>[2x]MEICPAVKRDVDLFLTGTPDEYVEQVAQYKALPVVLE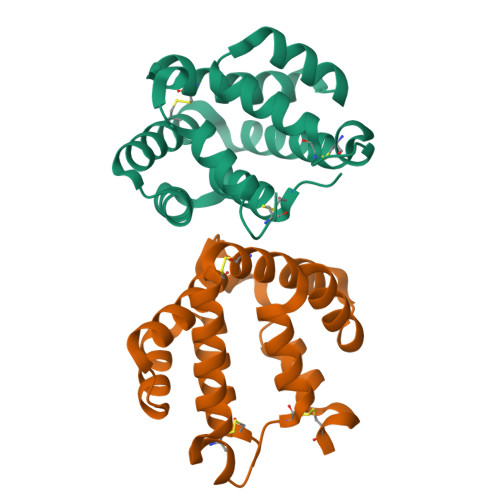NARILKNCVDAKMTEEDKENALSLLDKIYTSPLCVKMAETCPIFYDVFFAVANGNELLLDLSLTKVNATEPERTAMKKIQDCYVENGLISRVLDGLVMTTISSSKDCMGEHHHHHH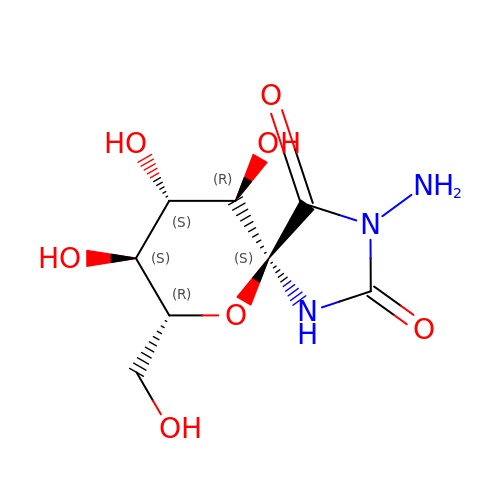(5S,7R,8S,9S,10R)-3-amino-8,9,10-trihydroxy-7-(hydroxymethyl)-6-oxa-1,3-diazaspiro[4.5]decane-2,4-dione | C8 H13 N3 O7 | KLJXQBRQPPSXPZ-WWHASAIZSA-N> GPGKQKPRYEIRWRVIESISPDGHEYIYVDPMQLPYDSRWEFPRDGLVLGRVLGSGAFGKVVEGTAYGLSRSQPVMKVAVKMLKPTARSSEKQALMSELKIMTHLGPHLNIVNLLGACTKSGPIYIIIEYCFYGDLVNYLHKNRDSFLSHKKKSMLDSEVKNLLSDDNSEGLTLLDLLSFTYQVARGMEFLASKNCVHRDLAARNVLLAQGKIVKICDFGLARDIMHDSNYVSKGSTFLPVKWMAPESIFDNLY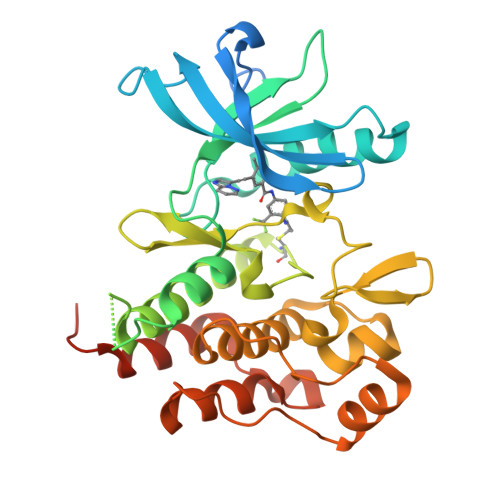TTLSDVWSYGILLWEIFSLGGTPYPGMMVDSTFYNKIKSGYRMAKPDHATSEVYEIMVKCWNSEPEKRPSFYHLSEIVENLLPGQYKKSYEKIHLDFLKSD>GSHMSTITRPIIELSNTFDKIAEGNLEAEVPHQNRADEIGILAKSIERLRRSLKQLADDRTLLMAGVSHDLRTPLTRIRLATEMMSEQDGYLAESINKDIEECNAIIEQFIDYLRT[2x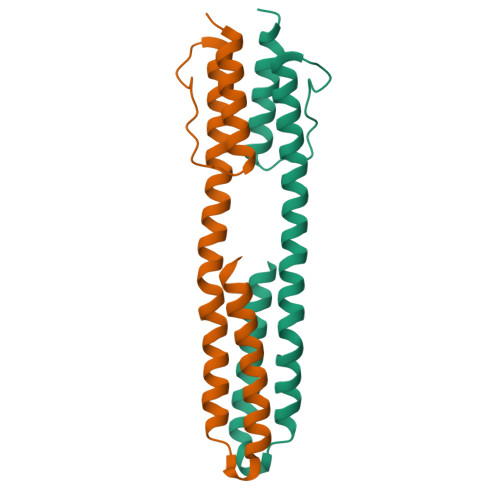]> RKTYTLTDYLKNTYRLKLYSLRWISDHEYLYKQENNILVFNAEYGNSSVFLENSTFDEFGHSINDYSISPDGQFILLEYNYVK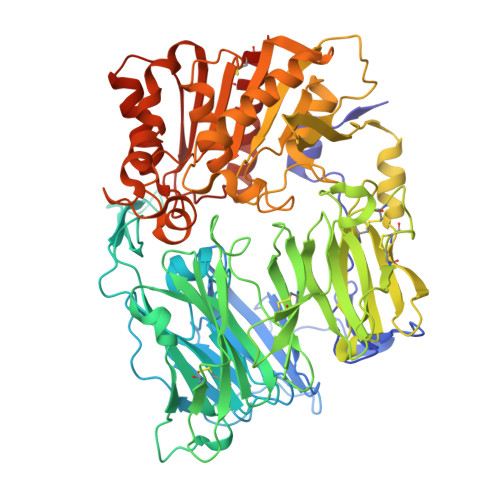QWRHSYTASYDIYDLNKRQLITEERIPNNTQWVTWSPVGHKLAYVWNNDIYVKIEPNLPSYRITWTGKEDIIYNGITDWVYEEEVFSAYSALWWSPNGTFLAYAQFNDTEVPLIEYSFYSDESLQYPKTVRVPYPKAGAVNPTVKFFVVNTDSLSSVTNATSIQITAPASMLIGDHYLCDVTWATQERISLQWLRRIQNYSVMDICDYDESSGRWNCLVARQHIEMSTTGWVGRFRPSEPHFTLDGNSFYKIISNEEGYRHICYFQIDKKDCTFITKGTWEVIGIEALTSDYLYYISNEYKGMPGGRNLYKIQLSDYTKVTCLSCELNPERCQYYSVSFSKEAKYYQLRCSGPGLPLYTLHSSVNDKGLRVLEDNSALDKMLQNVQMPSKKLDFIILNETKFWYQMILPPHFDKSKKYPLLLDVYAGPCSQKADTVFRLNWATYLASTENIIVASFDGRGSGYQGDKIMHAINRRLGTFEVEDQIEAARQFSKMGFVDNKRIAIWGWSYGGYVTSMVLGSGSGVFKCGIAVAPVSRWEYYDSVYTERYMGLPTPEDNLDHYRNSTVMSRAENFKQVEYLLIHGTADDNVHFQQSAQISKALVDVGVDFQAMWYTDEDHGIASSTAHQHIYTHMSHFIKQCFSLP> MAIETNAVVITDLNPLYPRD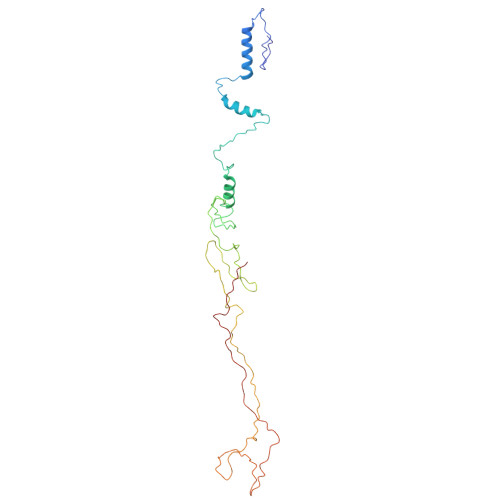RDYIYEGAAQIRLIKQTLQNTFPNVTEPVDIDSDTFKIMSEKLKFTGDAMDVGGLMIKNVTPGTGDKDVVTKGQMEAFMKNWMENKLYRIGSYYITEEDINPGDSISLGFGSWAKVTGVIMGTGVVNPDGSVPNAQRVEFQAGGTGGRVFNTIRTENVPLMTVNGSSFSLSSNTHSHNMVFGRGDASGHNSSPNWYSPGGGYSQRTDNDTHTHTISGSVSLGRDDISRQPINTLPPFRAAHIWRRIS>MAQLSVEQFLNEQKQAVETALSRYIERLEGPAKLKKAMAYSLEAGGKRIRPLLLLSTVRALGKDPAVGLPVACAIEMIHTYSLIHDDLPSMDNDDLRRGKPTNHKVFGEAMAILAGDG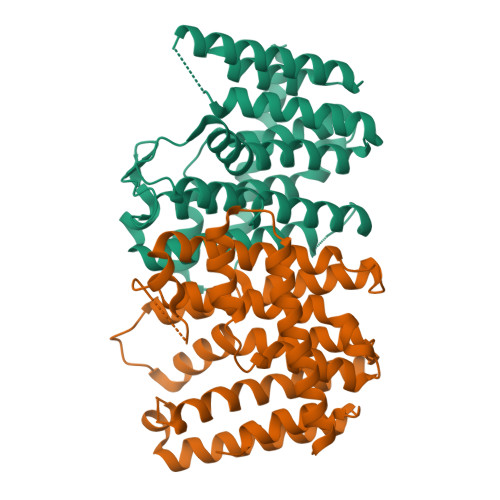LLTYAFQLITEIDDERIPPSVRLRLIERLAKAAGPEGMVAGQAADMEGEGKTLTLSELEYIHRHKTGKMLQYSVHAGALIGGADARQTRELDEFAAHLGLAFQIRDDILDIEGAEEKIGKPVGSDQSNNKATYPALLSLAGAKEKLAFHIEAAQRHLRNADVDGAALAYICELVAARDH[2x]>[2x]MEGGPALFQSDMTFKIFIDGEVNGQKFTIVADGSSKFPHGDFNAHAVCETGKLPMSWKPICHLIQYGEPFFARYPDGISHFAQECFPEGLSIDRTVRFENDGTMTSHHT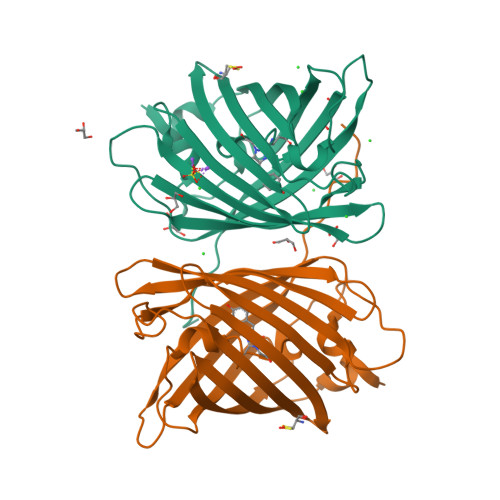YELDDTCVVSRITVNCDGFQPDGPIMRDQLVDILPNETHMFPHGPNAVRQLAFIGFTTADGGLMMGHFDSKMTFNGSRAIEIPGPHFVTIITKQMRDTSDKRDHVCQREVAYAHSVPRITSAIGSDED>[2x]LAFNEPLNVVSHLNHDWFLFGDSRSDCNHINNLKIKNFDYLDIHPSLCNNGKISSSAGDSIFKSFHFTRFYNYTGEGDQIIFYEGVNFNPYHRFKCFPNGSNDVWLLNKVRFYRALYSNMAFFRYLTFVDIPYNVSLSKFNSCKSDILSLNNPIFINYSKEVYFTLLGCSLYLVPLCLFKSNFSQYYYNIDTGSVYGFSNVVYPDLDCIYISLKPGSYKVSTTAPFLSLPTKALCFDKSKQFVPVQVVDSRWNNERASDISLSVACQLPYCYFRNSSANYVGKYDINHGDSGFISILSGLLYNVSCISYYGVFLYDNFTSIWPYYSFGRCPTSSIIKHPICVYDSDPLVPR

Human CoVs HKU1 and OC43 (subgenus Embecovirus, genus Betacoronavirus) are related but distinct. A second type of envelope protein unique to embecoviruses, called the haemagglutinin-esterase (HE), serves as a receptor-destroying enzyme. However, OC43 and HKU1, subject to convergent evolution, lost HE lectin function. In HKU1, HE lectin function was also lost, but here the LD underwent several deletions.

Here we present the structure of HKU1 HE at a global resolution of 3.4 Å. The quality of the map permitted modelling of residues 15–346. Each protomer is stabilised by six disulfide bonds, the presence of which are corroborated by the cryo-EM density. Dimerisation of HKU1 HE is achieved by interaction of the vestigial LDs and the membrane-proximal domains (MP). Indeed, comparison of the membrane-proximal domain and esterase domain of HKU1 to these related proteins revealed a high-level of structural conservation, with the aligned Cα positions having RMSD values of 0.81 Å and 0.76 Å for MCoV-New-Jersey strain (MCoV-NJ), and 0.83 Å and 0.84 Å for BCoV-Mebus strain. The lectin domain jelly roll core is essentially conserved in HKU1, with RMSD values of 0.95 Å and 0.89 Å for BCoV and MCoV-NJ, respectively. However, whereas in BCoV and MCoVs extensive loops emanate from this jelly roll core to form the LD carbohydrate-binding site (CBS), such loops are either much shorter or absent in the HKU1 HE structure. Thus, HKU1 has lost all essential components of the HE CBS and the LD domain has been stripped back essentially to the jelly roll core. Compared to related embecoviruses, the LD of HKU1 has four unique N-linked glycosylation sites: N110, N145, N168 and N193, two of which localise to the remnants of the elongated β5-β6 loop and β7-β10 loop. Interestingly, the disordered portion of these glycans forms a crown of glycan density, which encircles the LD and covers much of its surface.>GPGSNEFYLKTWSEWEKNGTPGEQRNIAFNRLKICLQNQEAELNLSELDLKTLPDLPPQITTLEIRKNLLTHLPDLPPMLKVIHAQFNQLESLPALPETLEELNAGDNKIKELPFLPENLTHLRVHNNRLHILPLLPPELKLLVVSGNRLDSIPPFPDKLEGLALANNFIEQLPELPFSMNRAVLMNNNLTTLPESVLRLAQNAFVNVAGNPLSGHTMRTLQQITTGPDYSGPRIFFSMG[2x];>GPGSEFQECAVCGWALPHNRMQALTSCECTICPDCFRQHFTIALKEKHITDMVCPACGRPDLTDDTQLLSYFSTLDIQLRESLEP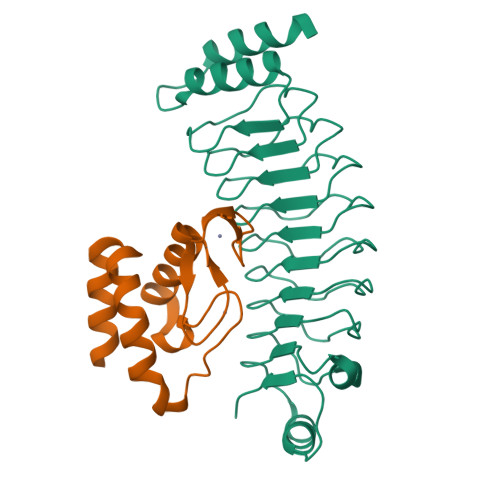DAYALFHKKLTEGVLMRD[2x]> KDSLRPKLSEEQQHIIAILLDAHHKTYDPTYADFRDFRPPVRMDG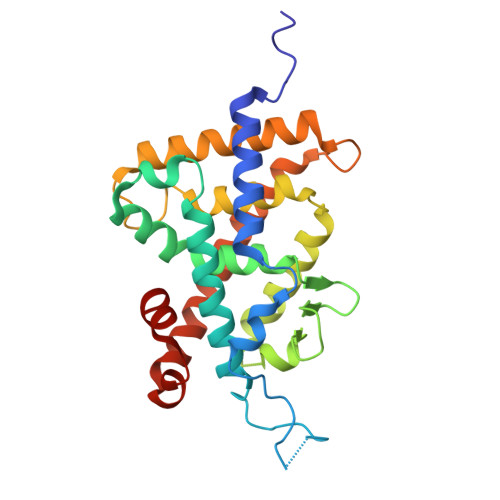STGSVTLDLSPLSMLPHLADLVSYSIQKVIGFAKMIPGFRDLTSDDQIVLLKSSAIEVIMLRSNQSFTMDDMSWDCGSQDYKYDVTDVSKAGHTLELIEPLIKFQVGLKKLNLHEEEHVLLMAICIVSPDRPGVQDAKLVEAIQDRLSNTLQTYIRCRHPPPGSHQLYAKMIQKLADLRSLNEEHSKQYRSLSFQPENSMKLTPLVLEVFG> MAAEVIEQHRRVILNEES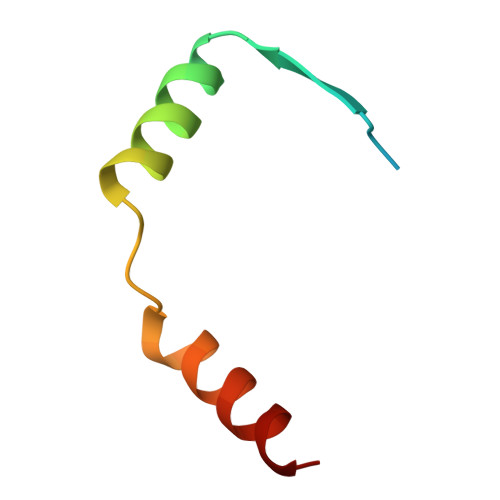WTRVMDALSNPPSPGEKLKRAAKRLQGM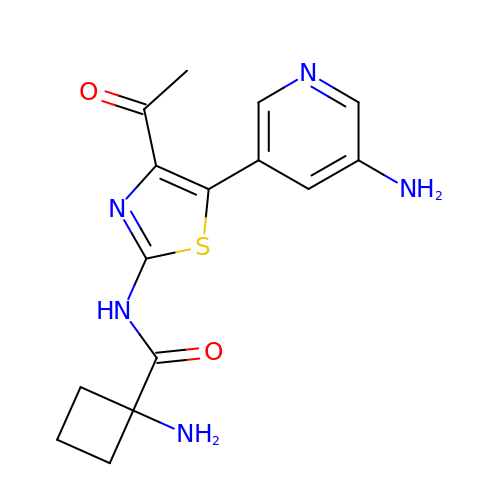1-azanyl-~{N}-[5-(5-azanylpyridin-3-yl)-4-ethanoyl-1,3-thiazol-2-yl]cyclobutane-1-carboxamide | C15 H17 N5 O2 S | KPPWHTAJUPKUOO-UHFFFAOYSA-N> MTIDEIIEAIEKLTVSELAELVKKLEDKFGVTAAAPVAVAAAPVAGAAAGAAQEEKTEFDVVLKSFGQNKIQVIKVVREITGLGLKEAKDLVEKAGSPDAVIKSGVSKEEAEE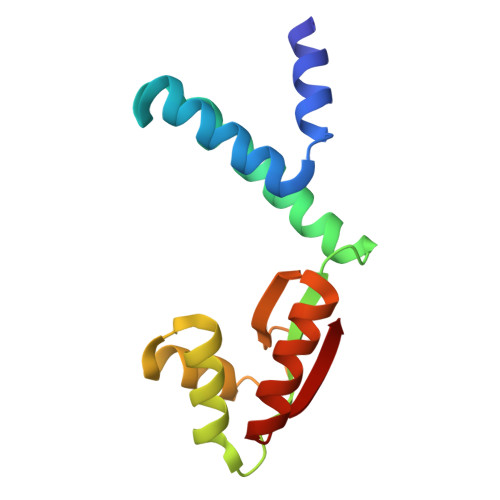IKKKLEEAGAEVELK> MVRVKVNDRIVEVPPGTSVMDAVFHAGYDVPLFCSEKHLSPIGACRMCLVRIGLPKKGPDGKPLLNEKGEPEIQWQPKLAASCVTAVADGMVVDTLSDVVREAQAGMVEFTLLNHPLDCPTCDKGGACELQDRTVEYGLYEKYYQKGPLELPVYTRFEFTRRHVDKHHPLSPFVILDRERCIHCKRCVRYFEEVPGDEVLDFIERGVHTFIGTMDFGLPSGFSGNITDICPVGALLDLTARFRARNWEMEETPTTCALCPVGCGITADTRSGELLRIRAREVPEVNEIWICDAGRFGHEWADQNRLKTPLVRKEGRLVEATWEEAFLA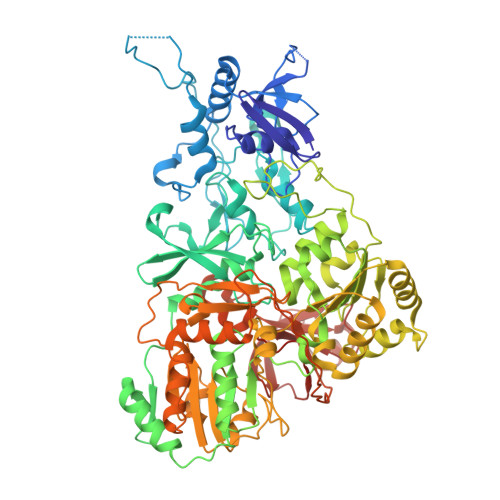LKEGLKEARGEEVGLYLAHDATLEEGLLASELAKALKTPHLDFQGRTAAPASLFPPASLEDLLQADFALVLGDPTEEAPILHLRLSEFVRDLKPPHRYNHGTPFADLQIKERMPRRTDKMALFAPYRAPLMKWAAIHEVHRPGEEREILLALLGDKEGSEMVAKAKEAWEKAKNPVLILGAGVLQDTVAAERARLLAERKGAKVLAMTPAANARGLEAMGVLPGAKGASWDEPGALYAYYGFVPPEEALKGKRFVVMHLSHLHPLAERYAHVVLPAPTFYEKRGHLVNLEGRVLPLSPAPIENGEAEGALQVLALLAEALGVRPPFRLHLEAQKALKARKVPEAMGRLSFRLKELRPKERKGAFYLRPTMWKAHQAVGKAQEAARAELWAHPETARAEALPEGAQVAVETPFGRVEARVVHREDVPKGHLYLSALGPAAGLRVEGRVLVPAGGEA5-[3-(6-methoxyisoquinolin-7-yl)-1H-pyrrolo[2,3-b]pyridin-5-yl]-N-methyl-N-prop-2-ynyl-pyridine-3-carboxamide | C27 H21 N5 O2 | 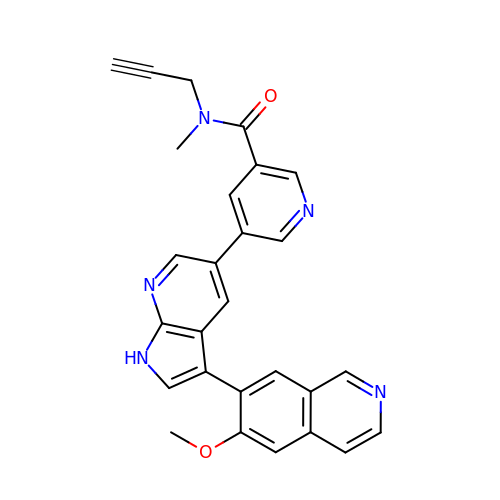QXTMJRCMHUDTRX-UHFFFAOYSA-N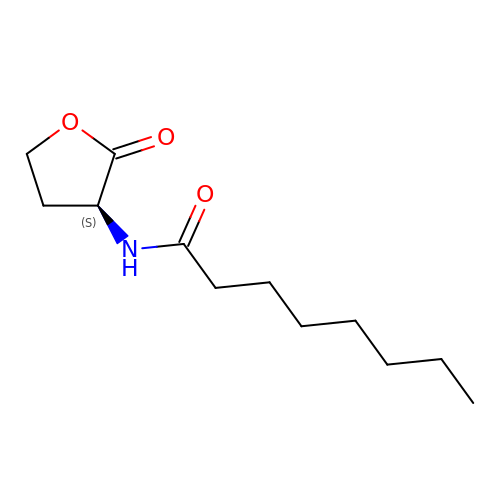N-(2-OXOTETRAHYDROFURAN-3-YL)OCTANAMIDE | C12 H21 N O3 | JKEJEOJPJVRHMQ-JTQLQIEISA-N OXA-48 confers resistance to many carbapenem and penicillin β-lactams, but only slowly hydrolyses oxyimino-cephalosporins such as ceftazidime (CAZ). Low catalytic activity for CAZ hydrolysis has been attributed to the substrate’s bulkiness, potentially requiring sampling of alternative loop conformations to promote cephalosporin binding and hydrolysis. Here we reveal how directed evolution of a β-lactamase yielded highly epistatic activity enhancements. We describe how distinct mutations shifted the rate-limiting step from substrate binding to the chemical reaction in the β-lactamase OXA-48, thereby causing strong phenotypic epistasis.

Five mutations accumulated along the evolutionary trajectory, F72L → S212A → T213A → A33V → K51E, resulting in Q5 conferring 43-fold increased CAZ resistance in Escherichia coli. The mutations acquired during evolution cluster around the active site or structural elements known to alter substrate specificity, such as the nucleophilic S70 or the Ω (D143–I164) and β5–β6 (T213–K218) loops. K51E increased resistance development by only 1.1-fold compared with Q4. Despite the introduction of S212A and T213A in the β5–β6 loop, the overall shape of this loop is preserved in Q5. Similarly, the overall active site architecture (for example, S70 and K73) was maintained in all variants. To estimate how the conformational dynamics changed during evolution, we performed ensemble refinements based on the crystal structures of wtOXA-48, F72L and Q5. Despite their differences in resolution, both F72L and Q5 revealed an increased flexibility primarily resulting in the Ω loop adopting various alternate conformations.

> EWQENKSWNVHFTEHKSQGVVVLWNENEQQGFTNNLKRANQAFLPASTLKIPNSLIALDLGVVKDEHQVFKWDGQTRDIATWNRDHNLITAMKYSVVPVYQEFARQIGEARMSKMLHAFDYGNEDISGNVDSFWLDGGIRISATEQISFLRKLYHNKLHVSERSQRIVKQAMLTEANGDYIIRAKTGYAARIEPKIGWWVGWVELDDNVWFFAMNMDMPTSDGLGLRQAITKEVLKQEKIIP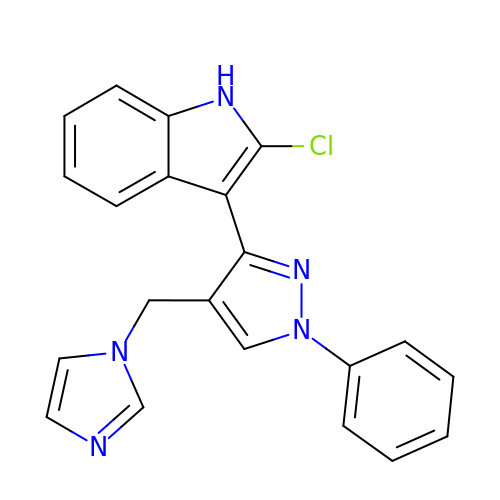2-chloranyl-3-[4-(imidazol-1-ylmethyl)-1-phenyl-pyrazol-3-yl]-1~{H}-indole | C21 H16 Cl N5 | RNSBGQRYBQOSEQ-UHFFFAOYSA-N>MRCIGISNRDFVEGVSGGSWVDIVLEHGSCVTTMAKNKPTLDFELIKTEAKQPATLRKYCIEAKLTNTTTESRCPTQGEPSLNEEQDKRFVCKHSMVDRGWGNGCGLFGKGGIVTCAMFRCKKNMEGKVVQPENLEYTVVITPHSGEEHAVGNDTGKHGKEVKITPQSSITEAELTGYGTVTMECSPRTGLDFNEMVLLQMENKAWLVHRQWFLDLPLPWLPGADTQGSNWIQKETLVTFKNPHAKKQDVVVLGSQEGAMHTALTGATEIQMSSGNLLFTGHLKCRLRMDKLQLKGMSYSMCTGKFKVVKEIAETQHGTIVIRVQYEGDGSPCKIPFEIMDLEKRHVLGRLITVNPIVTEKDSPVNIEAE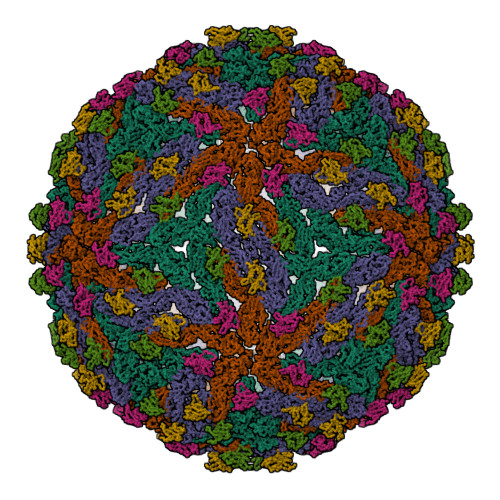PPFGDSYIIIGVEPGQLKLDWFKKG[3x];>FHLTTRNGEPHMIVSRQEKGKSLLFKTEDGVNMCTLMAMDLGELCEDTLTYKCPLLRQNEPEDIDCWCNSTSTWVTYGTCT[3x]> MMNAQKSKIALLLAASAVTMALTGCGGSDGNNGNDGSDGGEPAGSIQTLNLDITKVSYENGAPMVTVFATNEADMPVIGLANLEI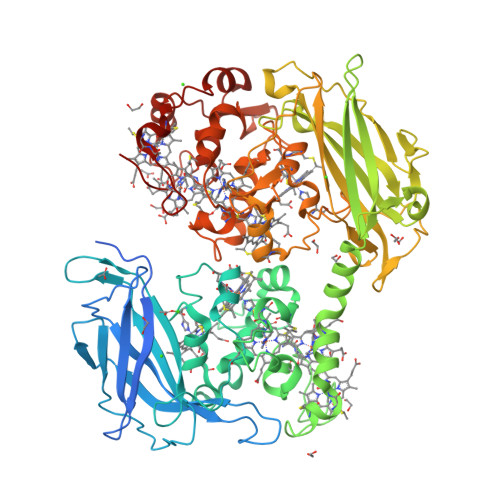KKALQLIPEGATGPGNSANWQGLGSSKSYVDNKNGSYTFKFDAFDSNKVFNAQLTQRFNVVSAAGKLADGTTVPVAEMVEDFDGQGNAPQYTKNIVSHEVCASCHVEGEKIYHQATEVETCISCHTQEFADGRGKPHVAFSHLIHNVHNANKAWGKDNKIPTVAQNIVQDNCQVCHVESDMLTEAKNWSRIPTMEVCSSCHVDIDFAAGKGHSQQLDNSNCIACHNSDWTAELHTAKTTATKNLINQYGIETTSTINTETKAATISVQVVDANGTAVDLKTILPKVQRLEIITNVGPNNATLGYSGKDSIFAIKNGALDPKATINDAGKLVYTTTKDLKLGQNGADSDTAFSFVGWSMCSSEGKFVDAADPAFDGVDVTKYTGMKADLAFATLSGKAPSTRHVDSVNMTACANCHTAEFEIHKGKQHAGFVMTEQLSHTQDANGKAIVGLDACVTCHTPDGTYSFANRGALELKLHKKHVEDAYGLIGGNCASCHSDFNLESFKKKGALNTAAAADKTGLYSTPITATCTTCHTVGSQYMVHTKETLESFGAVVDGTKDDATSAAQSETCFYCHTPTVADHTKVKM>GTSTQTKAGSLTIVGTGIESIGQMTLQALSYIEAAAKVFYCVIDPATEAFILTKNKNCVDLYQYYDNGKSRLNTYTQMSELMVREVRKGLDVVGVFYGHPGVFVNPSHRALAIAKSEGYRARMLPGVSAEDCLFADLCIDPSNPGCLTYEASDFLIRDRPVSIHSHLVLFQVGCVGIADFNFTGFDNNKFGVLVDRLEQEYGAEHPVVHYIAAMMPHQDPVTDKYTVAQLREPEIAKRVGGVSTFYIPPKARKASNLDIIRRLELLPAGQVPDKKARIYPANQWEPDVPEVEPYRPSDQAAIAQLADHAPPEQYQPLATSKAMSDVMTKLALDPKALADYKADHRAFAQSVPDLTPQERAALELGDSWAIRCAMKNMPSSLLDAARESGEEASQNG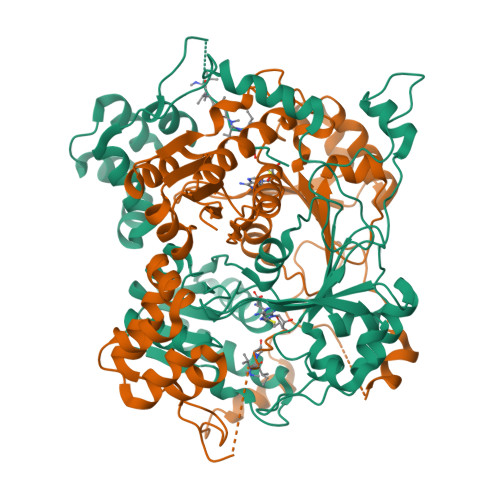FPWVIVVGVIGVIG[2x]>[3x]MGSDKIHHHHHHMEELLKELERIREEAKPLVEQRFEEFKRLGEEGTEEDLFCELSFCVLTANWSAE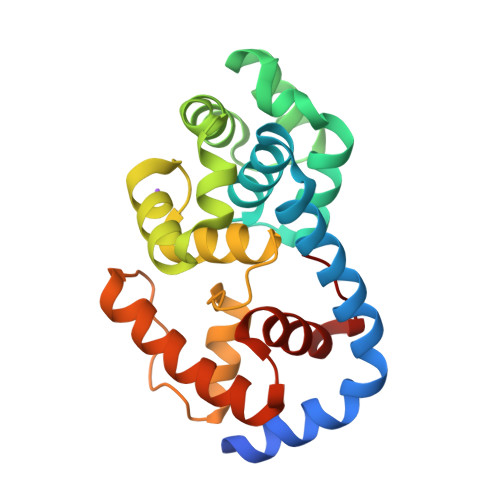GGIRAQKEIGKGFVHLPLEELAEKLREVGHRYPQKRAEFIVENRKLLGKLKNLVKGDPFQSREFLVRNAKGIGWKEASHFLRNTGVEDLAILDKHVLRLMKRHGLIQEIPKGWSKKRYLYVEEILRKVAEAFGESPGKFDLYLWYLVKGKVDK> CKGADGAHGVNGCPGTAGAAGSVGGPGCDGGHGG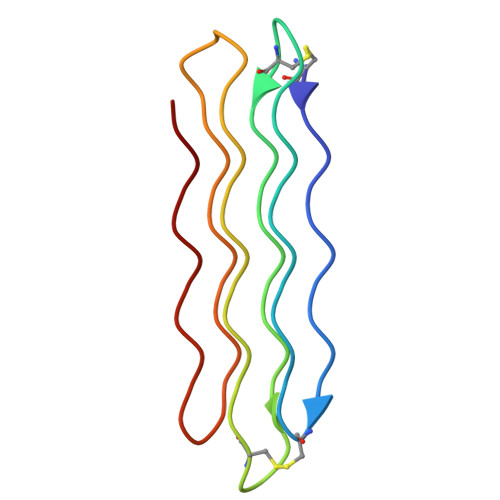NGGNGNPGCAGGVGGAGGASGGTGVGGRGGKGGSGTPKGADGAPGAP>[3x]MTMPNGSGGLDPGAWLSHWVNQADLSSLAGRTEDEVRAYFENLVQADSGWGDASNTFFNLILGGFQNLSEFVTLIVQAVTGAPGGLTDLQAFLTERWGDLADAFQAVANLIDAIAGEVGSSLADAIAKLATFLTELSPLNAGMLFGLIGTNHLPLLSVSHIANINPELLVNAGFDSDVSVVDNPYWDWDGTVGRTAPLGAVKVVADGTIKDLLSGPDAIPVVEGQKLNVSAWLK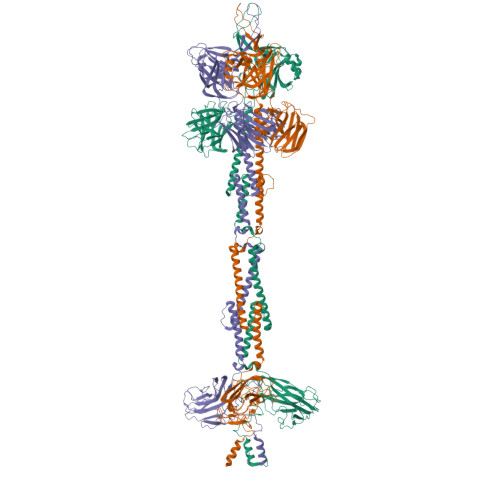YSGLVAGAGAGSIRLSGTAYSADGEVVAYPDFGGIPDGASGTSDWTQVTGQYVVPAGVTQFRLRLSVRENATGGTVWFDDCSVKKAGLLPQGLVDGLVQALSDLLTWLESLVDNVLSALGLDPIGTIVDKILDLADEFGDWLGATEDTAANLSNLLTKLLSDPASVIGPLAQSMITGLTGALGNLNTAINQIGDVLVGTVVTPINSAISNVIDWFNSLLNFQDTTTSNQINQQNFQIATLASGIKKQQWECRYSTAFVTFPEMFCDWGFALGGTTGAQSTGTAHTHTLNTDGLAALQIQILPAGYAIGGYIGISDTTIVDTIAMKMYKETSSAINNVYLEVFREDSTGALTSVGSVDVSGQLTTASDYVEATLPAGVIVNAGERYVVRMRNATTVGNRVGVSVMKELVGGRELSIRTETATDSNKTFYTPSEVLTAQGVSVIMPWAMMAAKNLATTDQSFSDDFNRSAMGGLWFLKSDTGTNQVGVSGGRAAFSGLTDGNQNALYIRPTAGDKQWVEATLYETGIAASGAREGLLMHANRDLSQVVYLGVNLNTAKIYTGPWNSLTERASVSTTGNDVLWQMYFDPATAAYTVLKNGQASGLTWTDSGSVVAHGPNYRFGGLRISRATFFNAGRIDNWTLKDWA>MMANRMILNETAWFGRGAVGALTDEVKRRGYQKALIVTDKTLVQCGVVAKVTDKMDAAGLAWAIYDGVVPNPTITVVKEGLGVFQNSGADYLIAIGGGSPQDTCKAIGIISNNPEFADVRSLEGLSPTNKPSVPILAIPTTAGTAAEVTINYVITDEEKRRKFVCVDPHDIPQVAFIDADMMDGMPPALKAATGVDALTHAIEGYITRGAWALTDALHIKAIEIIAGALRGSVAGDKDAGEEMALGQYVAGMGFSNVGVGLVHGMAHPLGAFYNTPHGVA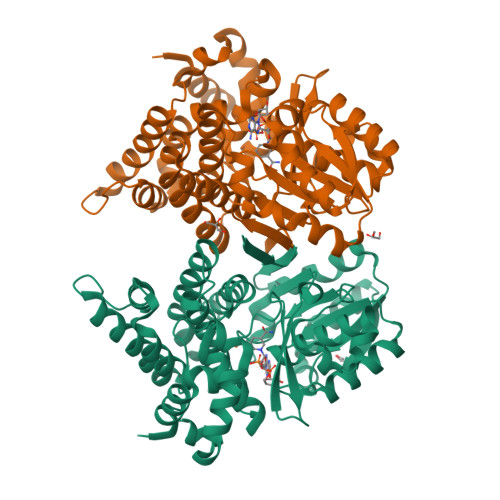NAILLPHVMRYNADFTGEKYRDIARVMGVKVEGMGLEEARNAAVEAVFALNRDVGIPPHLRDVGVRKEDIPALAQAALDDVCTGGNPREATLEDIVELYHTAWTSHHHHH[2x]>[2x]GENLLLPDLWLDFLQLSPIFQRKLAAVIACVRRLRTQATVYPEEDMCMAWARFCDPSDIKVVILGQDPYHGGQANGLAFSVAYGFPVPPSLRNIYAELHRSLPEFSPPDHGCLDAWASQGVLLLNTILTVQKGKPGSHADIGWAWFTDHVISLLSERLKA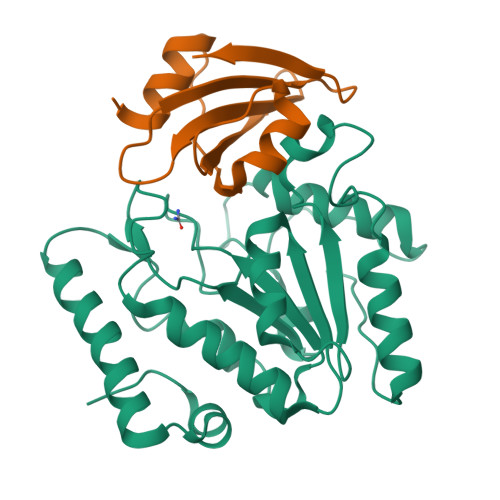CVFMLWGAKAGDKASLINSKKHLVLTSQHPSPLAQNSTRKSAQQKFLGNNHFVLANNFLREKGLGEIDWRL;>MTNLSDIIEKETGKQLVIQESILMLPEEVEEVIGNKPESDILVHTAYDESTDENVMLLTSDAPEYKPWALVIQDSNGENKIKML[2x]>MGNKICQFKLVLLGESAVGKSSLVLRFVKGQFHEFQESTIGAAFLTQTVCLDDTTVKFEIWDTAGQERYHSLAPMYYRGAQAAIVVYDITNEESFARAKNWVKELQRQASPNIVIALSGNKADLANKRAVDFQEAQSYADDNSLLFMETSAK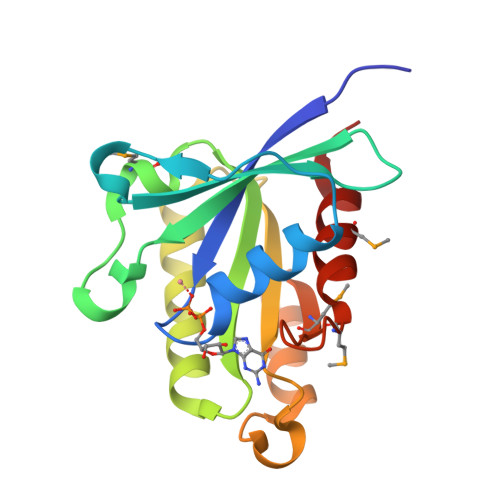TSMNVNEIFMAIAKKLPKN[4x]>[12x]EDPHLRNRPGKGHNYIDGMTQEDATCKPVTYAGACSSFDVLLEKGKFPLFQSYAHHRTLLEAVHDTIIAKADPPSCDLQSAHGNPCMKEKLVMKTHCPNDYQSAHYLNNDGKMASVKCPPKYELTEDCNFCRQMTGASLKKGSYPLQDLFCQSSEDDGSKLKTKMKGVCEVGVQALKKCDGQLSTAHEVVPFAVFKNSKKVYLDKLDLKTEENLLPDSFVCFEHKGQYKGKLDSGQTKRELKSFDISQCPKIGGHGSKKCTGDAAFCSAYECTAQYANAYCSHANGSGIVQIQVSGVWKKPLCVGYERVVVKRELS;>DPGCSELIQASSRITTCSTEGVNTKCRLSGTALIRAGSVGAEACLMLKGVKEDQTKFLKIKTVSSELSCREGQSYWTGSFSPKCLSSRRCHLVGECHVNRCLSWRDNETSAEFSFVGESTTMRENKCFEQCGGWGCGCFNVNPSCLFVHTYLQSVRKEALRVFNCIDWVHKLTLEITDFDGSVSTIDLGASSSRFTNWGSVSLSLDAEGISGSNSFSFIESPGKGYAIVDEPFSEIPRQGFLGEIRCNSESSVLSAHESCLRAPNLISYKPMIDQLECTTNLIDPFVVFERGSLPQTRNDKTFAASKGNRGVQAFSKGSVQADLTLMFDNFEVDFVGAAVSCDAAFLNLTGCYSCNAGARVCLSITSTGTGSLSAHNKDGSLHIVLPSENGTKDQCQILHFTVPEVEEEFMYSCDGDERPLLVKGTLIAID[12x]

Rift Valley fever virus (RVFV; genus phlebovirus, family Phenuiviridae) is an important example of an enveloped virus that harbours a class II fusion protein. As with other phleboviruses, RVFV displays two glycoproteins on the lipid bilayer envelope of the virion, Gn and Gc, which form higher order pentameric and hexameric ring-shaped assemblies. While the Gc glycoprotein is responsible for membrane fusion, the role of the Gn remains undefined. Virus entry is completed upon Gc-mediated fusion of the viral envelope and host cell membrane, in a pH-dependent mechanism.

Single-particle averaging and 3D reconstruction yielded a 13-Å resolution reconstruction of the Gn–Gc spike envelope. The resolution of the reconstruction was most likely limited to 13-Å due to remaining flexibility of the particles, despite efforts to include in the reconstruction only the most ordered particles by manual selection and 3D classification. The resolution was further improved by application of our localized reconstruction method, which accounted for the flexibility remaining in the fixed RVFV virions. We first performed fitting with the localized reconstruction of the pentamer at 7.7 Å resolution, followed by fitting the resulting Gn–Gc heterodimer model to localized reconstructions of the hexamers at 8.0–8.6 Å resolution. This sequential fitting approach allowed us to create a full atomic description of the Gn–Gc glycoprotein shell by applying icosahedral symmetry to the 12 Gn–Gc dimers in the asymmetric unit. Indeed, the improved resolution of the density maps for the capsomers reported here (7.7–8.6 Å), combined with high-resolution crystal structures, allowed the construction of an accurate atomic model of the whole virion surface. Consistent with previous biochemical and structural studies, this fitting verified that the Gn and Gc assemble as heterodimers, which form higher order ring-like pentameric and hexameric capsomer structures on the mature virion. Domain A of the Gn forms a ring on top of these capsomers interacting with domain II of Gc, occluding a surface area of ~950 Å2. The Gn–Gc interface is formed between the β-ribbon domain of the Gn and the hydrophobic fusion loops of Gc11, which are shielded from solvent at the interface between Gn domains A and B. Surprisingly, unlike the rod-like array of extended anti-parallel Gc dimers predicted from the low-resolution modelling attempts, we observed that RVFV Gc forms a kinked conformation, not previously sampled in crystallographic investigations of class II fusion glycoproteins. In toto, our integrative structural biology approach reveals the shielding of the Gc fusion loop in the pre-fusion state by its partner protein Gn.3-(2-methoxycarbonylphenyl)benzoic 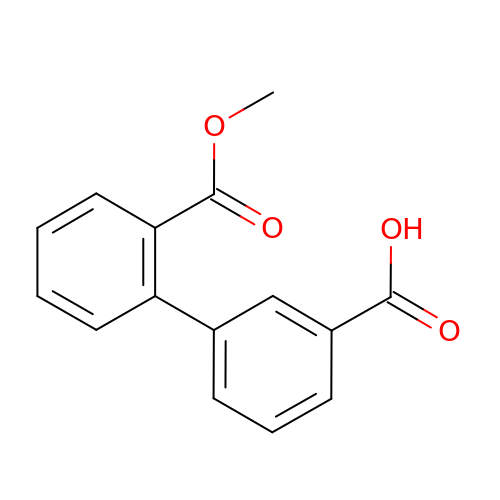acid | C15 H12 O4 | WUPZXYHQWDAHQT-UHFFFAOYSA-N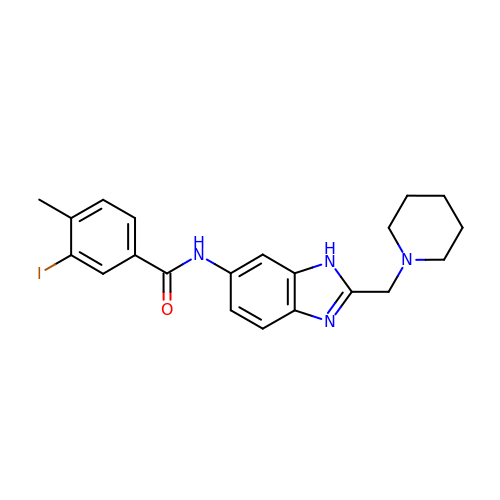3-iodanyl-4-methyl-~{N}-[2-(piperidin-1-ylmethyl)-3~{H}-benzimidazol-5-yl]benzamide | C21 H23 I N4 O | VMKBJIIRNPWSSI-UHFFFAOYSA-N N-[(1H-benzimidazol-2-yl)methyl]furan-2-carboxamide 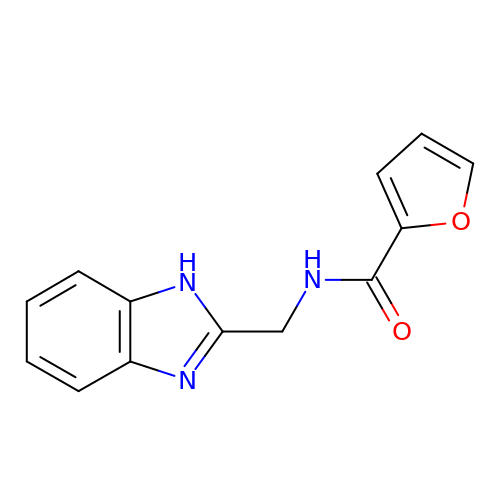| C13 H11 N3 O2 | WFEIYWNIMQWEHE-UHFFFAOYSA-N> DKYETNVSYKKLNQLAPYFKGFDGSFVLYNEREQAYSIYNEPESKQRYSPNSTYKIYLALMAFDQNLLSLNHTEQQWD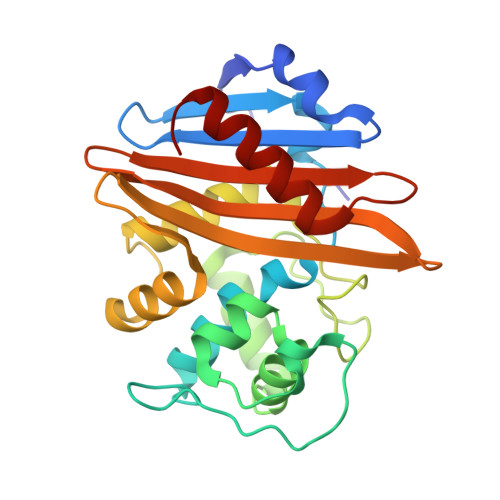KHQYPFKEWNQDQNLNSSMKYSVNWYYENLNKHLRQDEVKSYLDLIEYGNEEISGNENYWNESSLKISAIEQVNLLKNMKQHNMHFDNKAIEKVENSMTLKQKDTYKYVGKTGTGIVNHKEANGWFVGYVETKDNTYYFATHLKGEDNANGEKAQQISERILKEMELI> GAMADDEKNALPISKDGYIRVPKERVNVNLTSIKKLREKVDDSIHRELTDIFANLNYVGVVDEERRLAAIQHDLKLFLIDY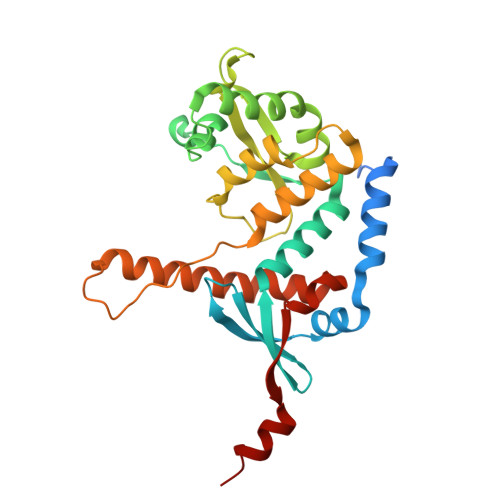GSVCYELFYQIGLTDFANFGKINLQSTNVSDDIVLYNLLSEFDELNDDASKEKIISKIWDMSSMLNEYYSIELVNDGLDNDLKSVKLKSLPLLLKGYIPSLVKLPFFIYRLGKEVDWEDEQECLDGILREIALLYIPDMVPKVDTSDASLSEDEKAQFINRKEHISSLLEHVLFPCIKRRFLAPRHILKDVVEIANLPDLYKVFERC>MAHHHHHHSSGLEVLFQGPDLHVIDHDFLKGQGDARSVRHIAIPAHRGLITDRNGEPLAVSTPVTTLWANPKELMTAKERWPQLAAALGQDTKLFADRIEQNAEREFIYLVRGLTPEQGEGVIALKVPGVYSIEEFRRFYPAGEVVAHAVGFTDVDDRGREGIELAFDEWLAGVPGKRQVLKDRRGRVIKDVQVTKNAKPGKTLALSIDLRLQYLAHRELRNALLENGAKAGSLVIMDVKTGEILAMTNQPTYNPNNRRNLQPAAMRNRAMIDVFEPGSTVKPFSMSAALASGRWKPSDIVDVYPGTLQIGRYTIRDVSRNSRQL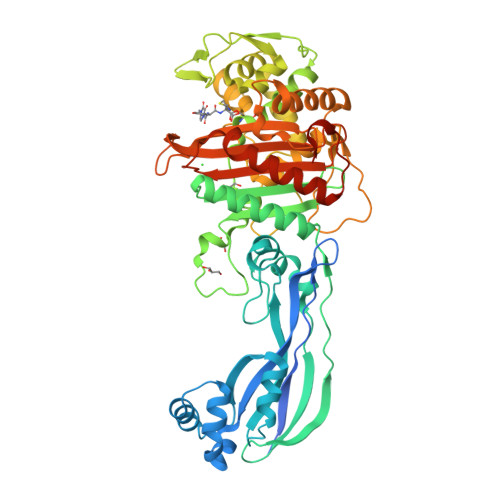DLTGILIKSSNVGISKIAFDIGAESIYSVMQQVGLGQDTGLGFPGERVGNLPNHRKWPKAETATLAYGYGLSVTAIQLAHAYAALANDGKSVPLSMTRVDRVPDGVQVISPEVASTVQGMLQQVVEAQGGVFRAQVPGYHAAGKSGTARKVSVGTKGYRENAYRSLFAGFAPATDPRIAMVVVIDEPSKAGYFGGLVSAPVFSKVMAGALRLMNVPPDNLPTATEQQQVNAAPAKGGRG[2x]5-(7-(5-HYDRO-4-METHYL-2-OXAZOLYL)PHENOXY)HEPTYL)-3-METHYL 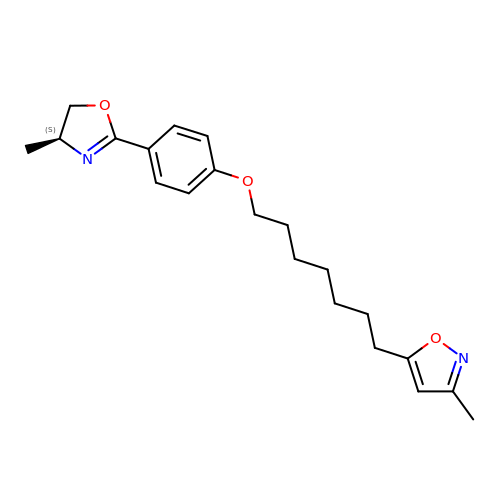ISOXAZOLE | C21 H28 N2 O3 | NEAZMARKCJKUMF-KRWDZBQOSA-N> MTVNWDINEALKNYMSDPSTIQTPEADSALVDCENDPESLLDNGLINSVLNPIVDAVAESPDAITRSHIFDSLQFLLKYTSYLSTHALSKLFDLITSGLGAEADVVHHDLESDEQELIPAHKQLLEMYGFLLQWTLTAAEAKAAEKSSTTVPARGRGKPKSKTGPGQDGTWDSVRQLETALSTMCKVLRLKLGKIFITTSERDTFIGLLTRPVYMILESEQRVKNTSIRMHAFKVLCMAVKHHGHGYAAQVSIVQNLTYFEHLSEPMAEFLHILAEQYDYPQLADEVLRELSNKEFNSNDTKGPKSVSAFMIRLSELAPRLVIKQVTLLAKQLDSESYTLRCALIEVFGNMLAYLSKSEERGENHKSQMNAFFDVLEERFLDINPYCRCRTIQVYIKLCELDQKFPKRRQRAAELACRSLMDKSSHVRRNAIKLLATLIRTHPFTALHGAQLARKDWQERLERVEAELNVLKPPPEAAGLEGDKANTSADQGLLDDATQVDSPKKRLEDMTEEEKIEAVRKAQEQAATSEAIEKLTLTKRYYTEALKFIDVLHEATPVICQLLGSKNKSEVIEAMDYFEIGDAYNIEQNKIGIRKMLRLIWTKGSSDEGKGVQTHLIECYKRLFFEAPDSFSPNDAANYIARNMISLTFGATPAELTSLEQLLHLMMKQGMIPDLVIAKLWQVYGVQRREISKKQRRGAIIVLGMLATASPEIVVGEMETMLRIGLGAHGRADLQLAKYTCIALRRINPTSRQTEKGSTTTFSRLPNDHAVLVKLAAITEVPTDNKEWYGVAEQAINAIYALSKHPDVLCSEIIRRKTRAVFARSTSKESVIGLSQLLFIVGHVAIKQIVHLELCELDFKRRKQEKDKEKAQQQEQEDNELDMIGGTTEDDFTEAMAHIRERELLFGPQSLLAQFGPMVSEICANNTVYKDRNLQQAATLCLAKLMCVSSEYCEANLPLLITIMERSPDPTVRSNAVIALGDMAVCFNHLIDENTDFLYRRLADPQPMVKRTCLMTLTFLILAGQVKVKGQLGEMAKCLEDEDKRIADLARMFFTELSTKDNAVYNHFVDMFSLLSADERIDEEAFRRIVRFLLGFVEKDKXXXXXXXXXXXXXXXXXXXXXXXXXXXXXXXXXXXXXXXXXXXXXXXXXXXXXX;> GHMEDGTVRKKPKKKTQRSSEATLAPSFASLQLKKLELEFAVDPFFKKASADFDEGGAKGLLLNHLMIDSQGRIVFDSSDDAEDVAEASAKPSREADDERPDSEDADADGDISMTDRDASAPGQVETQPEEEDEDVEIDVAALGAKYFPDLSILDSLDVCPSLKTFDLGDPSGSLYIPFLKVPDDWRHDQEKEKTPG

The condensin protein complex plays a key role in the structural organization of genomes. Based on their homology to ATP binding cassette (ABC) transmembrane transporters and the Rad50 DNA damage repair protein, the two globular ATPase “head” domains situated at the ends of ∼50-nm-long intra-molecular coiled coils of a heterodimer of condensin’s Smc2 and Smc4 subunits are thought to sandwich a pair of ATP molecules between composite catalytic sites, each composed of Walker A (P loop) and Walker B motifs of one head and a so-called ABC signature motif of the opposite head. Each head domain (hd) can be subdivided into a “RecA”-like lobe that contains the ATP-binding pocket and a “helical” lobe that merges into the coiled coils; they connect the heads to a half-doughnut-shaped “hinge” dimerization domain. Smc2hd and Smc4hd are furthermore connected by their binding to opposite ends of the Brn1Cnd2/NCAPH kleisin subunit (Onn et al., 2007).

Because Ycs4 has so far been thought to assemble into the condensin complex exclusively through its constitutive interaction with the Brn1 kleisin subunit (Onn et al., 2007, Piazza et al., 2014), we mapped the part of Ct Brn1 required for Ct Ycs4 binding to a high-affinity (Kd = 0.70 nM) core region of ∼175 residues (Ct Brn1336–512) and to an extended region that includes the preceding ∼110 residues (Ct Brn1225–512). To reveal the interaction between the Brn1 kleisin and Ycs4 HEAT-repeat subunits at near-atomic resolution, we solved the co-crystal structure of Ct Ycs4 bound to Ct Brn1225–418 to 3.3-Å resolution (Ct Ycs4-Brn1Y4). The structure revealed a hook-shaped conformation of the 21 HEAT-repeat motifs of Ycs4, with the low-affinity binding region of the kleisin subunit (Ct Brn1241–299) winding along the concave surface of the HEAT-repeat solenoid and entirely filling the space between the two lobes of the sharp U-turn in the C-terminal part of the Ycs4 subunit. A marked drop in the quality of the electron density map in the second lobe because of crystallographic disorder only allowed modeling of a polyalanine chain into unaccounted electron density alongside the tip of the Ycs4 U-turn, which presumably corresponds to the high-affinity kleisin core binding region. Localization of selenomethionine residues based on anomalous difference maps and secondary structure prediction nevertheless allowed the assignment of residue numbers for almost all of Ycs4. A feature apparently unique to Ycs4 is an α-helical extension of HEAT-repeat motif 10 (“proboscis”), which showed, however, no apparent primary sequence conservation among Ycs4 homologs.DEAH-box adenosine triphosphatases (ATPases) play a crucial role in the spliceosome-mediated excision of pre-mRNA introns. The catalytic activation, the catalysis itself as well as the final disassembly steps are driven by so-called DEAH-box helicases. They all belong to the helicase superfamily 2 (SF2) and share at least eight conserved sequence motifs (motifs I, Ia, Ib, II, III, IV, V and VI) spread over two RecA-like domains that together form the helicase core. Two RecA-like domains, referred to as RecA1 and RecA2, build up the helicase core. The RecA2 domain contains an anti-parallel β-hairpin present in all DExH-box helicases, which protrudes out of the RecA2 domain thereby contacting the C-terminal domains. These domains are divided in three distinct domains, namely the winged-helix (WH), the helix-bundle (HB) and the oligonucleotide-binding (OB) domain.

A structural analysis revealed that a serine in motif V is involved in polar interactions with one of the ligands in all structurally characterized catalytic states. Since mainly the mainchain of the motif V serine interacts via water-mediated hydrogen bonds with the adenosine nucleotides, we tested if a higher flexibility of the mainchain at this position has an effect on catalysis. We could furthermore structurally characterize Prp22-S837A in the adenosine nucleotide-free but RNA-bound state, as well as Prp43-S387A and Prp43-S387G in the ATP-bound state. Since Prp22 could not be crystallized in the presence of an ATP-analog, an existing crystallization condition for ADP-BeF3−-bound Prp43 was used to structurally characterize motif V serine mutants of a DEAH-box ATPase in this state. The structures of these three mutants show that motif V is able to adopt the same nucleotide-specific conformations regardless of the side chain property. In the ADP/ATP-bound structures, the mainchain of this residue interacts via hydrogen-bonds with conserved water molecules constituting the active site. The interactions in the ATP-bound state force the serine mainchain to adopt an unfavored conformation, enabling the mainchain nitrogen to hydrogen bond with the catalytic water. Instead, the mainchain is sufficient for sensing the adenosine nucleotide state at the active site and this sensing function is sensitive to the flexibility of the mainchain. While the ATP binding is improved at maximum flexibility (glycine), the sensing function is completely abolished at minimum flexibility (proline). The lack of a side chain at this residue position in motif V of other SF2 members is in agreement with the findings that it is dispensable for the function.

> GTTAKQAEAVEDSDINPWTGQRHSERYFKILKARRKLPVNKQRQEFLDLYHNNQILVFVGETGSGKTTQIPQYVLYDELPHQTGKLIACTQPRRVAAMSVAQRVADELDVKLGEEVGYSIRFENKTSSKTLLKYMTDGQLLREAMHDRDMSRYSCIILDEAHERTLATDILMALLKQLSERRKDLKIIVMSATLDAQKFQSYFFNAPLLAVPGRTHPVEIFYTPEAERDYVEAAIRTVLQIHACEPEGDILLFLTGEEEIEDACRRISLEVDEMIRESDAGPMSVYPLYGTLPPHQQQRIFEKAPQPFRPGGRPGRKCIVATNIAETGLTIDGIVYVVDPGFSKQKIYNPRTRVESLLVSPISKASAQQRAGRAGRTRPGKCFRLYTEEAFKKELIEQTYPEILRSNLSNTVLELKKLGVEDLVHFDLMDPPAPETMMRALEELNYLACLDDDGELTPLGNLASEFPLDPALAVMLISSPEFYCSNEILSITSLLSVPQIWVRPANARKRADEMKAQFAHPDGDHLTLLNAYHAYKGAEARGEDMKKWCHEHFLSYRHLSSADNVRAQLKKIMETHGIELVSTPFHDKNYYTNIRRALLAGFFMQVAMRESSNSKVYKTVKDEQLVLIHPSTTVTTPYEWVVYNEFVLTTKQYVRTVTNIRPEWLLEIAPVYYDLSTFQKGEIKNALTRVAEKIRRQQAMKASKA> EDLPHHDEKTWNVGSSNRNKAENLLRGKRDGTFLVRESSKQGCYACSVVVDGEVKHCVINKTATGYGFAEPYNLYSSLKELVLHYQHTSLVQHNDSLNVTLAYP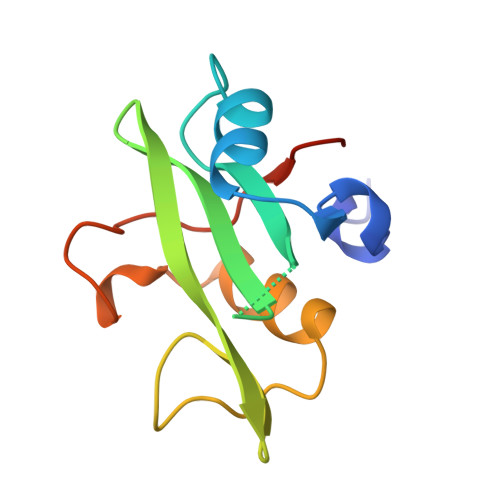VYAQQRR> AQSVPYGVSQIKAPALHSQGYTGSNVKVAVIDSGIDSSHPDLKVAGGASMVPSETNPFQDNNSHGTHVAGTVAALNNSIGVLGVAPSASLYAVKVL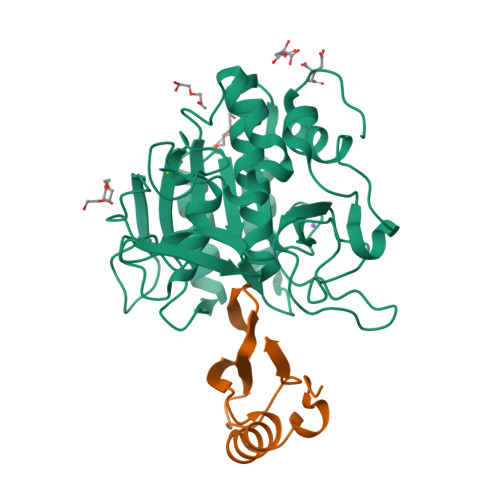GADGSGQYSWIINGIEWAIANNMDVINMSLGGPSGSAALKAAVDKAVASGVVVVAAAGNEGTSGSSSTVGYPGKYPSVIAVGAVDSSNQRASFSSVGPELDVMAPGVSIQSTLPGNKYGAYNGTSMASPHVAGAAALILSKHPNWTNTQVRSSLENTTTKLGDSFYYGKGLINVQAAAQHHHHHH;> MKTEWPELVGKSVEEAKKVILQDKPAAQIIVLPVGTIVTKEYRIDRVRLFVDRLDNIAQVPRVG> GAMALEARLEQASILKKVVDAIKDLVQDCNFDCNDSGIALQAMDNSHVALVSMMLKAEGFSPYRCDRNIALGVNLTSLTKVLRAAQNEDILTLKAEDAPD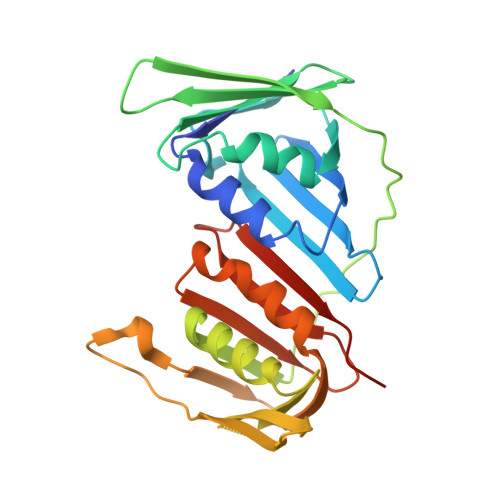VLNLVFESSETDRISEYDLKLMDIDQEHLGIPETEYAATITMPSNEFKRITTDLMAMSESVTIEANKDGVKFSCQGDIGNGSVTLRQHTNVEKPNESIEIELSEPVSLTFSLKYLVNFCKASALSNTVKICLSNEVPLLVEYSLGGSSYLRFYLAPKIGDDE> QADGAKIYAQCAGCHQQNGQGIPGAFPPLAGHVAEILAKEGGREYLILVLLYGLQGQIEVKGMKYNGVMSSFAQLKDEEIAAVLNHIATAWGDAKKVKGFKPFTAEEVKKLRAKKLTPQQVLAERKK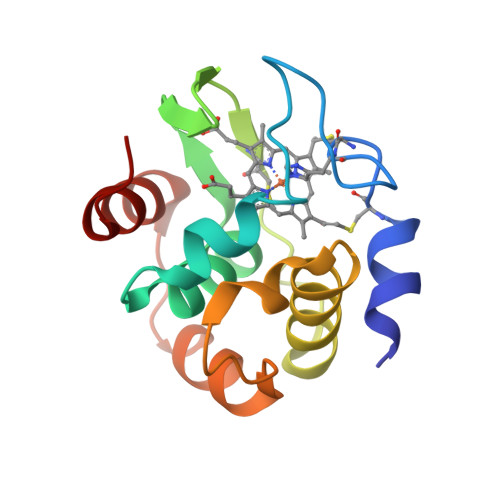LGLK Endoplasmic reticulum aminopeptidase 1 (ERAP1) cleaves the N-terminal amino acids of peptides, which can then bind onto major histocompatibility class I (MHC-I) molecules for presentation onto the cell surface, driving the activation of adaptive immune responses. Given that ERAP1-trimmed peptides modulate the adaptive immune response, controlling ERAP1 activity is an attractive strategy for cancer immunotherapy, autoimmune diseases and increasing immune responses against pathogens. Herein we describe the hit-to-lead optimization of a series of cyclohexyl acid ERAP1 inhibitors, found by X-ray crystallography to bind at an allosteric regulatory site. Binding of peptides to the regulatory site plays a critical role in determining ERAP1 substrate length requirements and the extent to which peptide trimming occurs through a “molecular ruler” mechanism.

Modified cyclohexane rings, such as sulfide 6 and difluorocyclohexane 7, resulted in further increases in potency. The binding modes of compound 7 (ERAP1 pIC50 = 7.7) and compound 13 (ERAP1 pIC50 = 8.6) largely overlaid well. As predicted for the FEP pose for compound 10, the most significant difference was in the orientation of the bicyclic ring, which presented the bromine atom and phenyl ring of compounds 7 and 13, respectively, into the lipophilic pocket. Comparing the two structures, there was also a significant movement of Gln730 to better fit the size and orientation of the ligand. To examine this selectivity, we tested compound 7, which was one of the most potent compounds in both the biochemical and cellular assays at the time. Pleasingly, 7 showed no measurable inhibition of ERAP2 or IRAP (pIC50 < 4.0, n = 1) and thus had >1,000-fold ERAP1 selectivity. In contrast, compound 7 had a significantly reduced unbound in vivo clearance with both good oral exposure and bioavailability. Furthermore, compound 7 demonstrated a much lower in vitro intrinsic clearance in rat and human hepatocytes, is 10-fold less lipophilic than compound 13, and has a much higher FaSSIF solubility. Furthermore, compound 7 had promising pharmacokinetic properties in rats, providing an excellent starting point for further optimization, which will be the subject of future publications.

> MVFLPLKWSLATMSFLLSSLLALLTVSTPSWCQSTEASPKRSDGTPFPWNKIRLPEYVIPVHYDLLIHAQLTTLTFWGTTKVEITASQPTSTIILHSHHLQISRATLRKGAGERLSEEPLQVLEHPRQEQIALLAPEPLLVGLPYTVVIHYAGQLSETFHGFYKSTYRTKEGELRILASTQFEPTAARMAFPCFDEPAFKASFSIKIRREPRHLAISNMPLVKSVTVAEGLIEDHFDVTVKMSTYLVAFIISDFESVSKITKSGVKVSVYAVPDKINQADYALDAAVTLLEFYEDYFSIPYPLPKQDLAAIPDFQSGAMENWGLTTYRESALLFDAEKSSASSKLGITMTVAHELAHQWFGNLVTMEWWNDLWLNEGFAKFMEFVSVSVTHPELKVGDYFFGKCFDAMEVDALQSSHPVSTPVENPAQIREMFDDVSYDKGACILNMLREYLSADAFKSGIVQYLQKHSYKNTKNEDLWDSMASIGSGGVDVKTMMNTWTLQRGFPLITITVRGRNVHMKQEHYMKGSDGAPDTGYLWHVPLTFITSKSDMVHRFLLKTKTDVLILPEEVEWIKFNVGMNGYYIVHYEDDGWDSLTGLLKGTHTAVSSNDRASLINNAFQLVSIGKLSIEKALDLSLYLKHETEIMPVFQGLNELIPMYKLMEKRDMNEVETQFKAFLIRLLRDLIDKQTWTDEGSVSERMLRSQLLLLACVHNYQPCVQRAEGYFRKWKESNGQLSLPVDVTLAVFAVGAQSTEGWDFLYSKYQFSLSSTEKSQIEFALCRTQNKEKLQWLLDESFKGDKIKTQEFPQILTLIGRNPVGYPLAWQFLRKNWNKLVQKFELGSSSIAHMVMGTTNQFSTRTRLEEVKGFFSSLKENGSQLRCVQQTIETIEENIGWMDKNFDKIRVWLQSEKLERMENLYFQ>[3x]DFSIVGYSQDDLTSTERLIQLFNSWMLNHNKFYENVDEKLYRFEIFKDNLNYIDETNKKNNSYWLGLNEFADLSNDEFNEKYVGSLIDATIEQSYDEEFINEDIVNLPENVDWRKKGAVTPVRHQGSCGSCWAFSAVATVEGINKIRTGKLVELSEQELVDCERRSHGCKGGYPPYALEYVAKNGIHLRSKYPYKAKQGTCRAKQ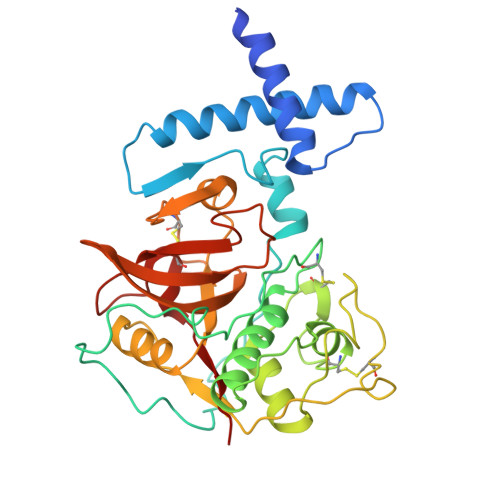VGGPIVKTSGVGRVQPNNEGNLLNAIAKQPVSVVVESKGRPFQLYKGGIFEGPCGTKVDGAVTAVGYGKSGGKGYILIKNSWGTAWGEKGYIRIKRAPGNSPGVCGLYKSSYYPTKN>GSHMDASVMSTTYALSAAQTEIWLAQQLYPDSPVYNIAQYTVIEGVIEPAVFEAALRQVIDEADTLRLQFIDSDDGLRQRIGTPAWSMPVLDLTAQADPQAAAQAWMRADYQQPVNLTQGPLFCYALLKVAPAQWMWYQRYHHIMMDGYGAYLIAQRVAYVYSALCEGTTPAECDFGSILQLLESDAQYQISAQRAQDEAYWLKHCANWSEPATLASRSAPVLQQRLRQTTYLAIQALGDTAPDARRLAQFMTAAMAAYLYRFTGEQDVVLGLPVKVRFGADRHIPGMKSNTLPLRLTMRPGMNLSSLMQQAAQEMQSGLRHQRYPSEALRRQLGMPSGQRLFGTTVNVMPFDLDLSFGGYSATNHNLLNGPAEDLMLGVYWTPGSHQLRIDFDANPACYTPEGLGAHQRRFIRFMQVLAADATQPIDSIDLLD[4x]

Nonribosomal peptide synthetases (NRPSs) are multimodular enzymes that catalyze the biosynthesis of diverse peptides with a wide variety of activities. The incorporation of an acyl into peptidyl backbone is usually implemented by a starter condensation (Cs) domain, normally located at the beginning of the initial NRPS module, via the formation of an amide bond to the α-amino group of the first amino acid residue, a process also known as lipoinitiation. Genome mining of two Cs domain-embedded cryptic NRPS biosynthetic gene clusters, rzmA and holA, in the bacterium P. rhizoxinica HKI 454 resulted in the discovery of two distinct types of lipopeptides, cyclic rhizomide A (1) containing an uncommon acetyl chain (C2) and linear holrhizin A (2) harboring a medium octanoyl (C8) chain. Similar to other C domain structures reported previously, RzmA-Cs adopts a “V-shaped” configuration and consists of two subdomains (N- and C-lobes) each representing the chloramphenicol acetyltransferase (CAT) fold.

We found that compared with wild-type (WT) RzmA, mutations at R148 indeed altered the production profile of rhizomide in vivo. A similar trend, but in the reverse direction could be seen for the HolA A149 mutations, in which longer residue side chains led to shorter acyl chains. These synchronized changes showed that the length of the side-chain of this key amino acid (R148 in RzmA-Cs, A149 in HolA-Cs) might control the length of acyl chains. The side-chain may act as an entry gate to a potential pocket. Therefore, truncating the side-chain of this residue could give a correspondingly deeper space for the extension of longer acyl-CoAs. After our initial attempts to cocrystallize WT RzmA-Cs with acyl-CoAs of various lengths failed, we noticed that the R148A mutant protein showed strong binding to C8-CoA, as evidenced by the high ΔTm in protein thermal shift assays and a Kd value of ~300 nM measured using isothermal titration calorimetry (ITC). Thus we selected this mutant for crystallization, and successfully obtained both unbound and C8-CoA-bound structures. The unbound R148A structure is mostly identical to that of WT RzmA-Cs in two conformations.SAHases (EC 3.3.1.1) catalyze the reversible hydrolysis of S-adenosyl-L-homocysteine (SAH), an important metabolite in the context of cellular methyltransferase regulation, to adenosine (Ado) and L-homocysteine (Hcy). SAHase is a potential pharmacological target, as abnormal levels of SAH can lead to pathological conditions, such as cardiovascular diseases. As reported by Manszewski et al. (2017), BeSAHase can adopt three different conformations, closed, open, and semi-open, which are defined by the relative orientation of the two major domains, the substrate-binding domain (where the Ado1 site is located) and the cofactor-binding domain (in the present structure marked by Ado2). Apart from the relative positions of the substrate- and cofactor-binding domains (here referred to as conformation), BeSAHase has another structural determinant, a molecular gate that controls access to a channel leading to the active site.

BeSAHase crystallized only when 10 and Ado were present simultaneously, whereas the protein incubated with 10 only did not form any crystals. The crystal belongs to the monoclinic space group P21, which is at variance with the orthorhombic system and P21212 space group that are characteristic of all previously determined BeSAHase structures. The present structure reveals a tetrameric assembly, which can be considered as a dimer of intimate dimers (AB and CD), even though the enzyme was deprived of NAD+ (because of the prior cofactor removal procedure). Indeed, the fact that no residual amounts of NAD+ were found in the electron density map confirmed the efficiency of the cofactor removal procedure with ammonium sulfate treatment. Although the molar excess over apo-enzyme was the same (12-fold) for both compounds (10 and Ado), only Ado molecules were found in the electron density maps. Interestingly, each BeSAHase subunit accommodated two Ado molecules. One is located in the typical Ado binding site in the substrate-binding domain (hereafter referred to as Ado1), forming the same hydrogen bonding network as in the previously reported structures. The other site (hereafter referred to as Ado2) coincides with the position that was previously shown to be occupied by the adenosine moiety of the NAD+ cofactor in the holo-enzyme (Manszewski et al., 2015, 2017). Otherwise, Ado2 is coordinated by Lys467 of the neighboring subunit (which uses its Nζ atom to form hydrogen bonds with O2′ and O3′ of the ribose moiety, with average bond lengths of 2.99 and 2.73 Å, respectively) in the same way as seen for the equivalent moiety of NAD+. The side chains of His342, however, adopt an orientation of the O state that has not been observed before.

>GIDPFTMNAKPGFTDYIVKDIALADFGRKEISLAETEMPGLMATREEYGPKQPLKGARIAGSLHMTIQTAVLIETLAALGADIRWVSCNIYSTQDHAAAAIAAAGIPVFAVKGETLTEYWDYTAKLFDWHGGGTPNMILDDGGDATMLVHAGYRAEQGDTAFLDKPGSEEEEIFYALVKRLLKEKPKGWFAEIAKNIKGVSEETTTGVHRLYEMANKGTLLFPAINVNDSVTKSKFDNLYGCRESLVDGIRRGTDVMLSGKVAMVAGFGDVGKGSAASLRQAGCRVMVSEVDPICALQAAMEGYEVVTMEDAAPRADIFVTATGNKDIITIEHMRAMKDRAIVCNIGHFDNEIQIASLRNLKWTNIKPQVDEIEFPDKHRIIMLSEGRLVNLGNAMGHPSFVMSASFTNQTLAQIELFANNKDSKYAKKVYVLPKTLDEKVARLHLAKIGVKLTELRKDQADYIGVKQEGPYKSDHYRY[4x]>[2x]GIVLFVDFDYFYAQVEEVLNPSLKGKPVVVCVFSGRFEDSGAVATANYEARKFGVKAGIPIVEAKKILPNAVYLPMRKEVYQQVSSRIMNLLREYSEKIEIASIDEAYLDISDKVRDYREAY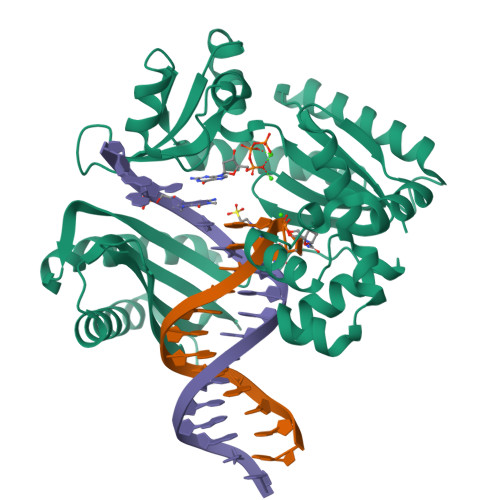NLGLEIKNKILEKEKITVTVGISKNKVFAKIAADMAKPNGIKVIDDEEVKRLIRELDIADVPGIGNITAEKLKKLGINKLVDTLSIEFDKLKGMIGEAKAKYLISLARDEYNEPIRTRVRKSIGRIVTMKRNSRNLEEIKPYLFRAIEESYYKLDKRIPKAIHVVAVTEDLDIVSRGRTFPHGISKETAYSESVKLLQKILEEDERKIRRIGVRFSKFI>MPGRRKACFVTALTSRTELDIDPDKLRESVVELLERHPLVFEGTRQLALQHRPEATDPWYEGCQRQSLISSDSDFTEVHGELRDTYLGEVFDRLPFKPIRTRIMALDPKYCYSVHRDLTPRYHLAVTTSEHARFVFIEHDKVLHIPADGDLYYVDTRQLHSAFNGGDDMAIHIVF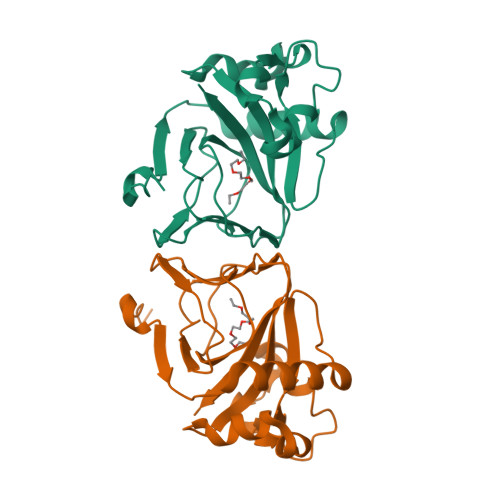GTDGESK[2x]N~1~-(1-propyl-1,3-dihydro-2H-benzimidazol-2-ylidene)benzene-1,3-dicarboxamide 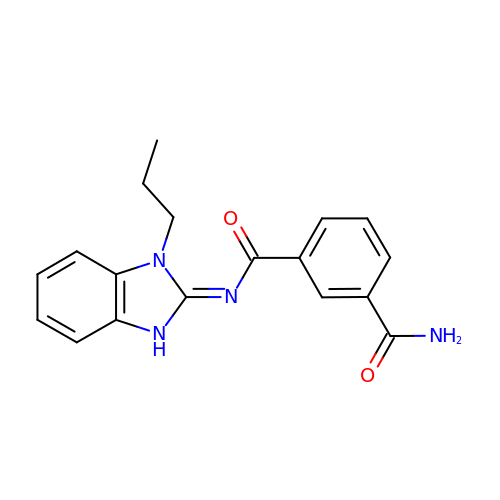| C18 H18 N4 O2 | UOZVVPXKJGOFIG-UHFFFAOYSA-N> SLVSDDKKDTGTIEIIAPLSGEIVNIEDVPDVVFAEKIVGDGIAIKPTGNKMVAPVDGTIGKIFETNHAFSIESDSGVELFVHFGIDTVELKGEGFKRIAEEGQRVKVGDTVIEFDLPLLEEKAKSTLT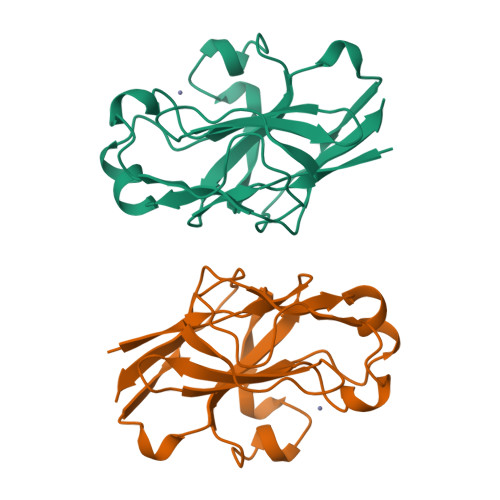PVVISNMDEIKELIKLSGSVTVGETPVIRIKK>RSCIDTIPKSRCTAFQCKHSMKYRLSFCR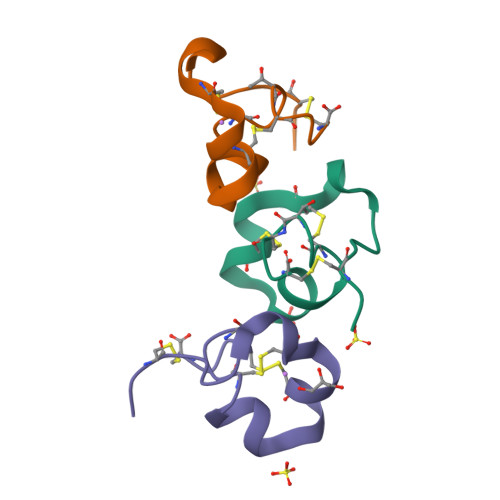KTCGTC[3x]>MGSSHHHHHHSQDPNSSSMTLGHMVQKAKESSGDVTPKKYNIFLASKPVDGDRKWLDVTNKYTNDVAAKVPQATHKDIDDAIDAAVAAAPAMAAMGAYERKAVLEKVVAELKNRFEEIAQTLTMESGKPIKDARGEVTRTIDTFQVAAEESVRIYGEHIPLDISARNKGLQGIVKKFPIGPVSMVSPWNFPLNLVAHKVAPAIAVGCPFVLKPASRTPLSALILGEILHKIEELPLGAFSILPVSREDADMFTVDERFKLLTFTGSGPIGWDMKARAGKKKVVMELGGNAPCIVDDYVPDLDYTIQRLINGGFYQGGQSCIH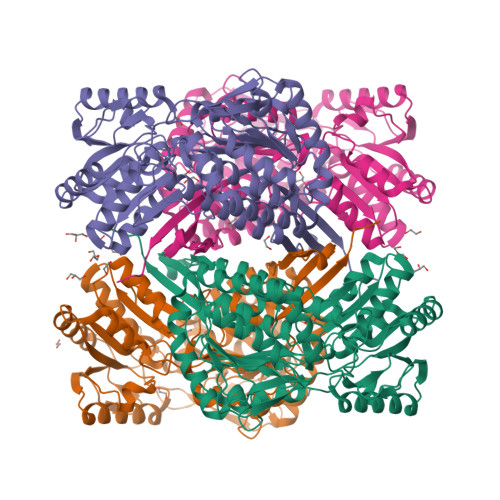MQRLYVHERLYDEVKEGFVAAVKKLKMGNPFEEDTYLGPMISESAAKGIEDWVKEAVAKGGKLLTGGNRKGAFIEPTVIEDVPIEANARKEEIFGPVVLLYKYSDFKEAVKECNNTHYGLQSGIFTKDLNKAFYAFEHMEVGGVILNDSPALRVDSQPYGGLKDSGIQREGVKYAMDDMLETKVLVMRNVGTL[4x]>[4x]SPNPLDVSKTYPTLHILLQFNHRGLEARIFRHGQLWAETHAEVVLRSKTKQISFLSNGSYPSMDATTPLNPWKSTYQAVLRAEPHRVTMDVYHKRIR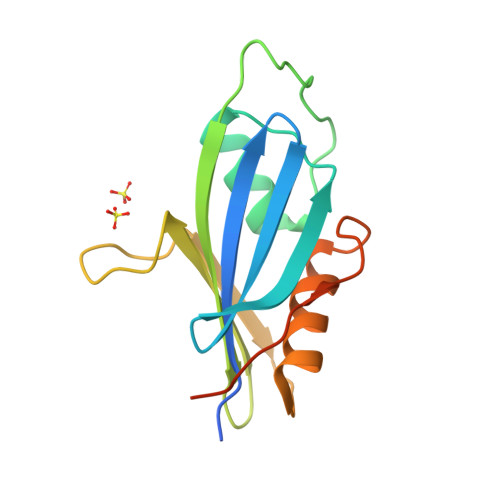PFRLPLVQKEWRTCEENVFGLYHVFETHYAGYFSDLLIHDVETNPGGSKHHHHHH Titin is the largest protein in nature extending from the Z-disk to the M-band, and interacts with a number of sarcomeric and signalling proteins. One of these targets is another giant myofibril-associated protein, termed obscurin (OBSCN), that interacts with titin at both the M-band and the Z-disk. Obscurin and titin also interact at the Z-disk, through Ig58/Ig59 of obscurin and the titin ZIg9/ZIg10. The Ig59 domain is only a part of the titin binding region; both obscurin Ig58 and Ig59 domains and both titin ZIg9 and ZIg10 domains are necessary for this interaction at the Z-disk.

We first solved the high-resolution structure of Ig59 (residues 4428–4521). Human obscurin Ig59 was isolated based on the original sequence alignment (CAC44768.1). The resulting structure shows beta sheets extending from Glu 4436 to Lys 4439 (strand A), Ala 4441 to Arg 4444 (strand A’), Ala 4445 to Thr 4454 (strand B), Ser 4465 to Ile 4469 (strand C), Trp 4480 to Asp 4485 (stand D), His 4488 to Leu 4494 (strand E), Gly 4502 to Ala 4507 (stand F), and Ala 4513 to Leu 4520 (strand G). Overall, the structure forms a typical Ig-like fold. Independently, the NMR solution structure of human obscurin Ig59 was solved with greater than 12 restraints per residue. The best NMR structure, as defined as that with the lowest RMSD, and X-ray structure are highly similar to each other, with a pairwise RMSD of 1.609 Å. Based on the evidence that mutations in the M10 domain of TTN, which binds the Ig1 of obscurin, are found in patients with muscular dystrophy we sequenced the OBSCN exons encoding the titin-binding region at both M-band and Z-disk of patients with a clinical history of molecularly undiagnosed distal dystrophy. This analysis revealed the presence of a heterozygous missense variant c.13330C>T in exon 51 predicting an amino acid change from arginine to tryptophan (p.Arg4444Trp) in the Ig59 of obscurin (according to sequence NP_443075) in the proband of a French family (Fig 2A individual III:3). The p.Arg4444Trp mutation could affect the obscurin-titin interaction in one of two ways: it may unfold the entire Ig59 domain, or it may maintain the fold and simply perturb the binding event. Circular dichroism (CD) experiments on the normal and mutant versions of the Ig59 domain are virtually identical, suggesting that the mutation does not globally disrupt the overall Ig-like architecture.

> RLEILELLKNAAVRAGAQACFTCTLSEAVPVGEASWYINGAAVQPDDSDWTVTADGSHHALLLRSAQPHHAGEVTFACRDAVASARLTVLGGLEHHHHHH>[3x]MKTYYEQDANVGLLQGKTVAVIGYGSQGHAQAQNLRDSGVEVVVGVRPGKSFEVAKADGFEVMSVSEAVRTAQVVQMLLPDEQQAHVYKAEVEENLREGQMLLFSHGFNIHFGQINP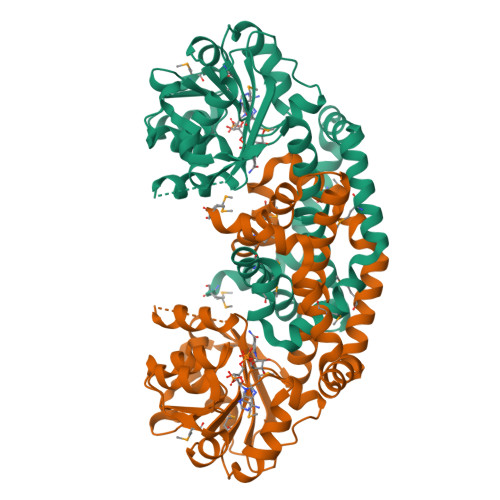PSYVDVAMVAPKSPGHLVRRVFQEGNGVPALVAVHQDATGTALHVALAYAKGVGCTRAGVIETTFQEETETDLFGEQAVLCGGVTALVKAGFETLTEGGYRPEIAYFECLHELKLIVDLMYEGGLTNMRHSISDTAEFGDYVTGSRIVTDETKKEMKRVLTEIQQGEFAKKWILENQAGRPTYNAMKKAEQNHQLEKVGEELREMMSWIHAPKELVKK>[2x]SNAMNQTLLSDFGTPVERVERAIDALRNGRGVMVLDDESRENEGDMVFAAEAMTLEQMALTIRHGSGIVCLCITDERRQQLDLPMMVTHNSSQFQTAFTVTIEAAEGVTTGVSAAD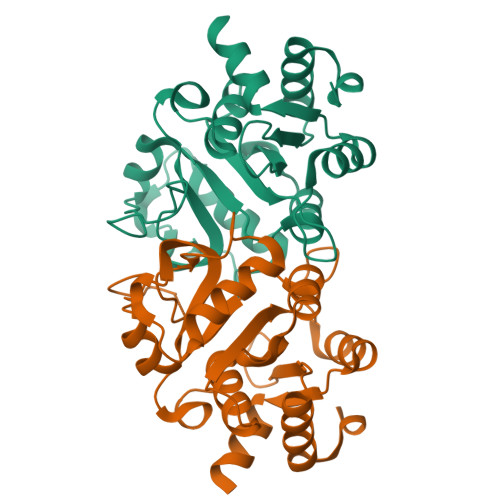RLTTIRKAIADNAKPADLNRPGHVFPLRGQPGGVLSRRGHTEASIDLATLAGYKPAGVLCELTNDDGSMAHAPEVIAFAKLHDMPVVTIDDLAAYLQSRAKKAS>MAILTDENYVDKAERAISLLEKDNKGNYLLTTSQIRKLLSLCSSLYDRSKERKFDELINDVSYLRVQFVYQAGREIAVKDLIEKAQILEALKEIKDRETLQRFCRYMEALVAYFKFYGGKD[3x];>[5x]MTFAKIKFSAQIRLETGLHIGGSDAFAAIGAIASPVIKDPITNIPIIPGSSLKGKMRTLLAKVYNEKVAEKPSDDSDILSRLFGNSKDKRFKMGRLIFRDAFLSNADELDSLGVRSYTEVKFENTIDRITAEANPRQIERAIRNSTFDFELIYEITDENENQVEEDFKVIRDGLKLLELDYLGGSGSRGYGKVAFEKLKATTVFGNYDVKTLNELLTAEV;> MTYKLYIMTFQNAHFGSGTLDSSKLTFSADRIFSALVLESLKMGKLDAFLAEANQDKFTLTDAFPFQFGPFLPKPIGYPKHDQIDQSVDVKEVRRQAKLSKKLQFLALENVDDYLNGELFENEEHAVIDTVTKNQPHKDGNLYQVATTRFSNDTSLYVIANESDLLNELMSSLQYSGLGGKRSSGFGRFELDIQNIPLELSDRLTKNHSDKVMSLTTALPVDADLEEAMEDGHYLLTKSSGFAFSHATNENYRKQDLYKFASGSTFSKTFEGQIVDVRPLDFPHAVLNYAKPLFFKLEV;> MKKEKIDLFYGALLHDIGKVIQRATGERKKHALVGADWFDEIADNQVISDQIRYHMANYQSDKLGNDHLAYITYIADNIASGVDRRQSNEESDEDASAKIWDTYTNQADIFNVFGAQTDKRYFKPTVLNLKSKPNFASATYEPFSKGDYAAIATRIKNELAEFEFNQAQIDSLLNLFEAILSFVPSSTNSKEIADISLAEHSRLTAAFALAIYDYLEDKGRHNYKEDLFTKASAFYEEEAFLLASFDLSGIQDFIYNIATSGAAKQLKARSLYLDFMSEYIADSLLDKLGLNRANLLYVGGGHAYFVLANTEKTVETLVQFEKDFNQFLLANFQTRLYVAFGWGSFAAKDIMSELNSPESYRQIYQKASRMISEKKISRYDYRTLMLLNRGGKSSERECEICHSVENLVSYHDQKVCDICRGLYQFSKEIAHDHFIITENEGLPIGPNACLKGVAFEKLSQESFSRVYVKNDYKAGTIKATHVFVGDYQCDEIHKYAALSKNEDGLGIKRLAVVRLDVDDLGAAFMAGFSRQGNGQYSTLSRSATFSRSMSLFFKVYINQFASDKKLSIIYAGGDDVFAIGSWQDIIAFTVELRQNFIKWTNGKLTLSAGIGLFADKTPISLMAHQTGELEEAAKGNEKDSISLF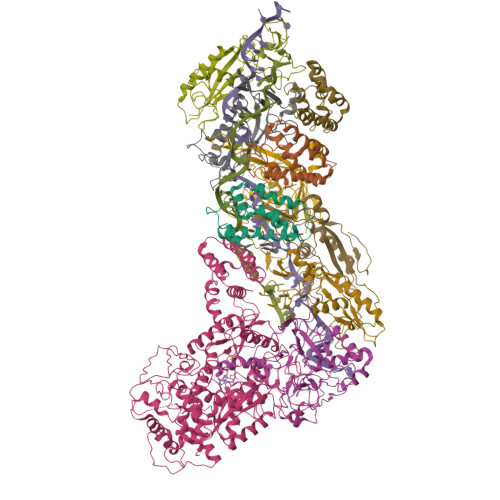SSDYTFKFDRFITNVYDDKLEQIRYFFNHQDERGKNFIYKLIELLRNYESEEKMNVARLAYYLTRLEELTDKDERDKFKQFKKLFFKWYTNNESDRKEAELALLLYVYEIRKD> MNNNKAEADTSSSMADPETRPTYTTHHLAIPSGVTQDEFDELKQSVVEFHTYQLSQNQCSSLLAQRIRAPNDVVWSIVRRFDQPQTYKHFIKSCSVSDNFTMAVGSTRDVNVISGLPAATSTERLDILDDDRQVTGFSIIGGEH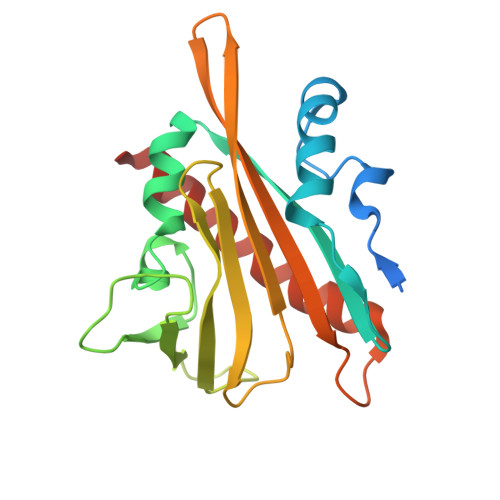RLRNYRSVTSVHGFNRDGAICTVVLESYVVDVPEGNTEEDTRLFADTVVKLNLQKLVSVAESQVI> MALSELALVRWLQESRRSRKLILFIVFLALLLDNMLLTVVVPIIPSYLYSIKHEKNATEIQTARPVHTASISDSFQSIFSYYDNSTMVTGNATRDLTLHQTATQHMVTNASAVPSDCPSEDKDLLNENVQVGLLFA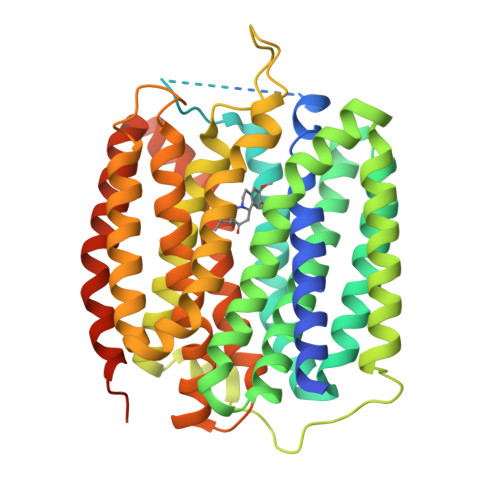SKATVQLITNPFIGLLTNRIGYPIPIFAGFCIMFVSTIMFAFSSSYAFLLIARSLQGIGSSCSSVAGMGMLASVYTDDEERGNVMGIALGGLAMGVLVGPPFGSVLYEFVGKTAPFLVLAALVLLDGAIQLFVLQPSRVQPESQKGTPLTTLLKDPYILIAAGSICFANMGIAMLEPALPIWMMETMCSRKWQLGVAFLPASISYLIGTNIFGILAHKMGRWLCALLGMIIVGVSILCIPFAKNIYGLIAPNFGVGFAIGMVDSSMMPIMGYLVDLRHVSVYGSVYAIADVAFCMGYAIGPSAGGAIAKAIGFPWLMTIIGIIDILFAPLCFFLRSPPSRLEEELRRRTEGGSSDLEVLFQ> VLQGTYVDGELNGPAQEYDTDGRLIFKGQYKDNIRHGVCWIYYPDGGSLVGEVNEDGEMTGEKIAYVYPDERTALYGKFIDGEMIEGKLATLMSTEEGRPHFELMPGNSVYHFDKSTSSCISTNALLPDPYESERVYVAESLISSAGEGLFSKVAVGPNTVMSFYNGVRITHQEVDSRDWALNGNTLSL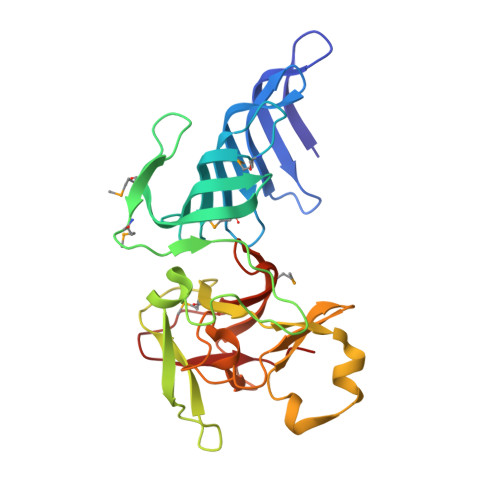DEETVIDVPEPYNHVSKYCASLGHKANHSFTPNCIYDMFVHPRFGPIKCIRTLRAVEADEELTVAYGY> EEMKKGHLERECMEETCSYEEAREVFED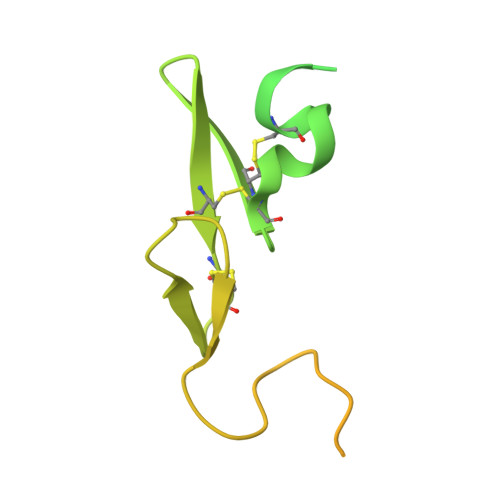SDKTNEFWNKYKDGDQCETSPCQNQGKCKDGLGEYTCTCLEGFEGKNCELFTRKLCSLDNGDCDQFCHEEQNSVVCSCARGYTLADNGKACIPTGPYPCGKQTLERRKRSVAQATSSSGEAPDSITWKPYDAADLDPTENPFDLLDFNQTQPERGDNNLTRIVGGQE>MGSSHHHHHHSQDPNSMPDNTIQWDKDADGIVTLTMDDPSGSTNVMNEAYIESMGKAVDRLVAEKDSITGVVVASAKKTFFAGGDVKTMIQARPEDAGDVFNTVETIKRQLRTLETLGKPVVAAINGAALGGGLEIALACHHRIAADVKGSQLGLPEVTLGLLPGGGGVTRTVRMFGIQNAFVSVLAQGTRFKPAKAKEIGLVDELVATVEELVPAAKAWIKEELKANPDGAGVQPWDKKGYKMPGGTPSSPGLAAILPSFPSNLRKQLKGAPMPAPRAILAAAVEGAQVDFDTASRIESRYFASLVTGQVAKNMMQAFFFDLQAINAGGSRPEGIGKTPIKRIGVLGAGMMGAGIAYVSAKAGYEVVLKDVSLEAAAKGKGYSEKLEAKALERGRTTQERSDALLARITPTADAADFKGVDFVIEAVFENQELKHKVFGEIEDIVEPNAILGSNTSTLPITGLATGVKRQEDFIGIHFFSPVDKMPLVEIIKGEKTSDEALARVFDYTLAIGKTPIVVNDSRGFFTSRVIGTFVNEALAMLGEGVEPASIEQAGSQAGYPAPPLQLSDELNLELMHKIAVATRKGVEDAGGTYQPHPAEAVVEKMIELGRSGRLKGAGFYEYADGKRSGLWPGLRETFKSGSSQPPLQDMIDRMLFAEALETQKCLDEGVLTSTADANIGSIMGIGFPPWTGGSAQFIVGYSGPAGTGKAAFVARARELAAAYGDRFLPPESLLS[2x];>MSEEAFIYE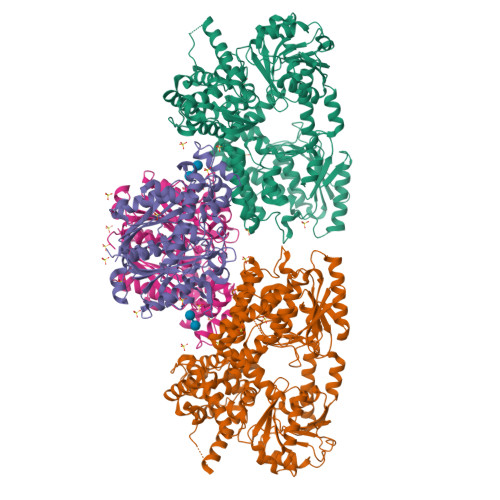AIRTPRGKQKNGSLHEVKPLSLVVGLIDELRKRHPDLDENLISDVILGCVSPVGDQGGDIARAAVLASGMPVTSGGVQLNRFCASGLEAVNTAAQKVRSGWDDLVLAGGVESMSRVPMGSDGGAMGLDPATNYDVMFVPQSIGADLIATIEGFSREDVDAYALRSQQKAAEAWSGGYFAKSVVPVRDQNGLLILDHDEHMRPDTTKEGLAKLKPAFEGLAALGGFDDVALQKYHWVEKINHVHTGGNSSGIVDGAALVMIGSAAAGKLQGLTPRARIVATATSGADPVIMLTGPTPATRKVLDRAGLTVDDIDLFELNEAFASVVLKFQKDLNIPDEKLNVNGGAIAMGHPLGATGAMILGTMVDELERRNARRALITLCIGGGMGVATIIERV[2x]> MQVLNTKSETKQENEGSQPPYIQERLKSLNDIETQLCSMLQEASQVTFIFGELKRGNESVKPQFENHVKQFYERLDKSTTQLRKEIQLLDENVGTRLLPINVNKKALGQDTEKMEEQLDLLSAILDPSKSK;> QEQFVKRRRDMLEHINLAMNESSLALEFVSLLLSSVKESTGMSSMSPFLRKVVKPSSLNSDKIPYVAPTKKEYIELDILNKGWKLQSLNESKDLLRASFNKLSSILQNEHDYWNKIMQSISNKDVIFKIRDRTSGQKLLAIKYGYEDSGSTYKHDRGIANIRNNIESQNLDLIPHSSSVFKGTDFVHSVKKFLRVRIFTKIESEDDYILSGESVMDRDSESEEAETKDIRKQIQLLKKIIFEKELMYQIKKECALLISYGVSIENENKVIIELPNEKFEIELLSLDDDSIVNHEQDLPKINDKRANLMLVMLRLLLVVIFKKTLRSRISSPHGLINLNVDDDILIIRPILGKVRFANYKLLLKKIIKDYVLDIVPGSSITETEVEREQPQENKNIDDENITKLNK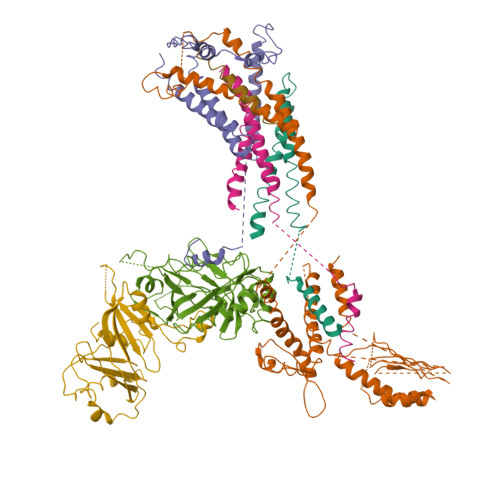EIRAFDKLLNIPRREXXXXXXXXXXXXXXXXXXXXXXXXXXXXXXXXXXXXXXXXXXXXXEVEDFLHFIVAEYIQQKKV;> MSQSTASLVPEGNQGSLQEDVSFDFNGVPGQALDAVRMRLAQLTHSLRRIRDEMSKAELPQWYTLQSQLNVTLSQLVSVTSTLQHFQETLDSTVVYPLPKFPTTSHESLVTTLLRKKNIPEVDEWMKYVRETSGVTTALLKDEEIEKLLQQDREITNWARTTFRNEYGKHDFKNEESLSEEHASLLVRDSKPSKPFNVDDVLKFTFTGEKPIITGSTSTSSSN;> MSNQALYEKLEQTRTILSVKLAELINMTTIADRNDDDEGSFAQENSELAVATTSVMMVNNQTMQLIKNVQDLLILTRSIKEKWLLNQIPVTEHSKVTRFDEKQIEELLDNCIETFVAEKTT;> MVQQLSLFGSIGDDGYDLLISTLTTISGNPPLLYNSLCTVWKPNPSYDVENVNSRNQLVEPNRIKLSKEVPFSYLIDETMMDKPLNFRILKSFTNDKIPLNYAMTRNINSDDIIDVDMDASPAPSNESCSPWSLQISDIPAAGNNRSVSMQTIAETIILSSAGKNSSVSSLMNGLGYVFEFQYLTIGVKFFMKHGLILELQKIWQIEEAGNSQITSGGFLLKAYINVSRGTDIDRINYTETALMNLKKELQGYIELSVPDRQSMDSRVAHGNILI;> MGKSAVIFVERATPATLTELKDALSNSILSVRDPWSIDFRTYRCSIKNLPADVSKLMYSITFHHHGRQTVLIKDNSAMVTTAAAADIPPALVFNGSSTGVPESIDTILSSKLSNIWMQRQLIKGDAGETLILDGLTVRLVNLFSSTGFKGLLIELQADEAGEFETKIAGIEGHLAEIRAKEYKTSSDSLGPDTSNEICDLAYQYVRALEL;> IFKIVQSRLMSTSYHLNSTLESLYD> SSLDDKPQFPGASAEFIDKLEFIQPNVISGIPIYRVMDRQGQIINPSEDPHLPKEKVLKLYKSMTLLNTMDRILYESQRQGRISFYMTNYGEEGTHVGSAAALDNTDLVFGQYREAGVLMYRDYPLELFMAQCYGNISDLGKGRQMPVHYGCKERHFVTISSPLATQIPQAVGAAYAAKRANANRVVICYFGEGAASEGDAHAGFNFAATLECPIIFFCRNNGYAISTPTSEQYRGDGIAARGPGYGIMSIRVDGNDVFAVYNATKEARRRAVAENQPFLIEAMTYRIGHHETSDDSSAYRSVD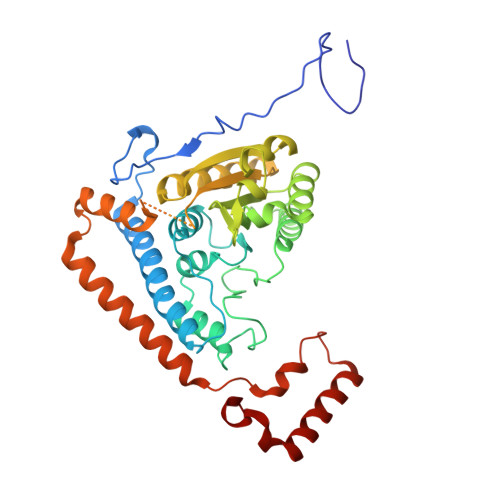EVNYWDKQDHPISRLRHYLLSQGWWDEEQEKAWRKQSRRKVMEAFEQAERKPKPNPNLLFSDVYQEMPAQLRKQQESLARHLQTYGEHYPLDHFDK>[2x]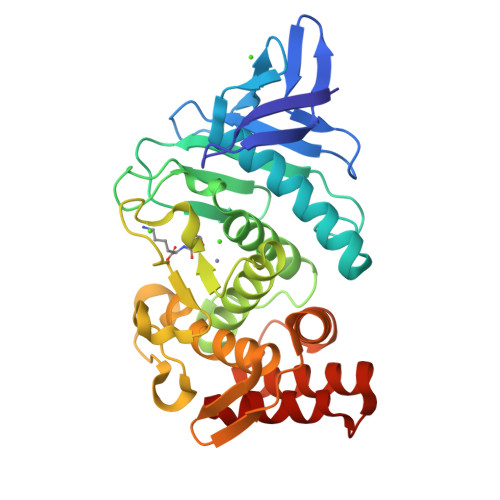ATGTGKGVLGDTKSFTTTASGSSYQLKDTTRGNGVVTYTASNRQSIPGTILTDADNVWNDPAGVDAHTYAAKTYDYYKAKFGRNSIDGRGLQLRSTVHYGSRYNNAFWNGSQMTYGDGDGSTFIAFSGDPDVVGHELTHGVTEYTSNLEYYGESGALNEAFSDVIGNDIQRKNWLVGDDIYTPNIAGDALRSMSNPTLYDQPDHYSNLYTGSSDNGGVHTNSGIINKAYYLLAQGGTFHGVTVNGIGRDAAVQIYYSAFTNYLTSSSDFSNARAAVIQAAKDQYGANSAEATAAAKSFDAVGVN> ACGTA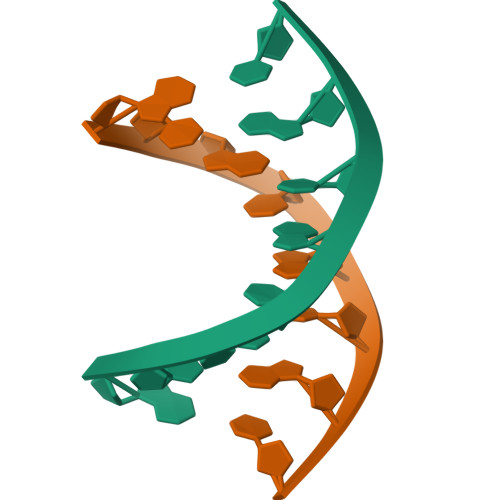CGT> XAEIAAIEYEQAAIKEEIAAIKDKI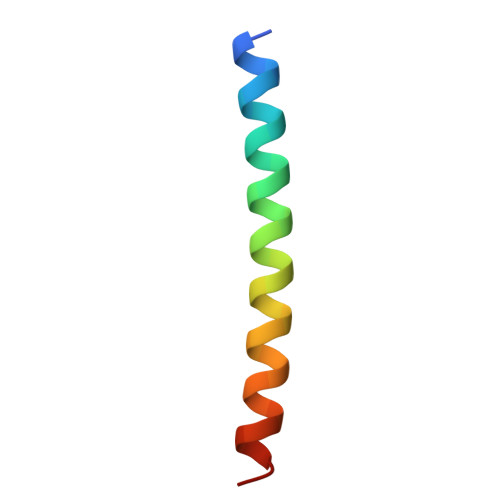AAIKEYIAAIX>[4x]VSNLIVNGTAENGMDGWPDWGYPVSAVPEAAYGGTKGFKLSGGKQAGMGQKVALKPNTTYILGAWGKFTAKPGTYCDVIVQYH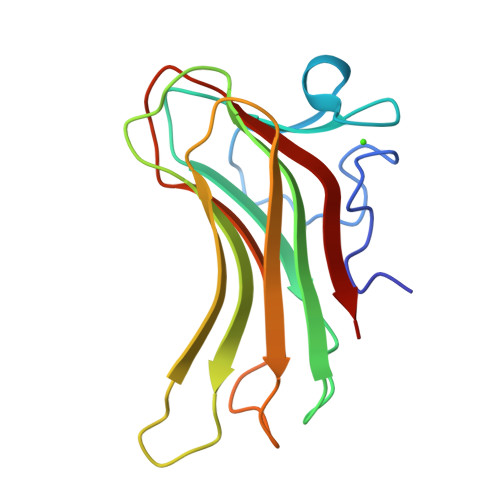LKDANNTYVQNILRFTETDWTYKQVVFTTPDAFGSDPEFVLWKDDASNADFYADNITLVEV>[2x]MEGEHQYLNLVREILERGVKKDDRTGTGTLSIFGPQMRFSLRDDTIPVLTTKKIFWRGVVEELLWFIRGNTDAKELAKKKIHIWNANGSREFLDSRGLYDRAE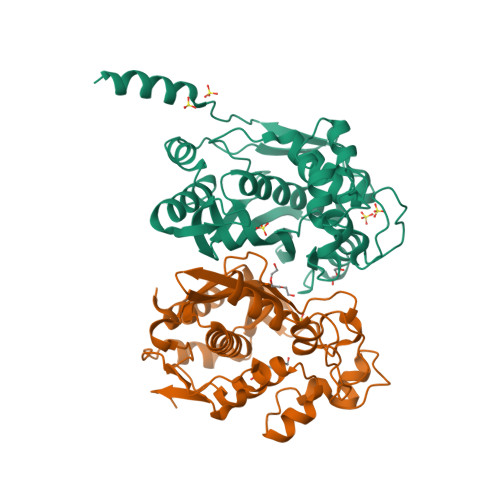GDLGPVYGFQWRHFGAEYDTCSSDYTGKGIDQLANILKTLRENPDDRRMIMTAWNPMDLHLMALPPCHMTAQFYVANGELSCQLYQRSGDVGLGVPFNIASYSLLTHLMASMVGLKPGEFILTLGDAHIYNTHIEVLKKQLCRVPRPFPKLRILMAPEKIEDFTIDMFYLEGYQPHSGNLQMKMAVLEHHHHHH Here structural analysis of hydroxyketoacid aldolase from Sphingomonas wittichii RW1 (SwHKA) revealed a dynamic movement of the metal cofactor between two coordination spheres without protein scaffold rearrangements. Holo‐SwHKA forms a trimer of homodimers, in which each monomer adopts an (α/β)8 triosephosphate isomerase (TIM) barrel fold. In total, holo‐SwHKA contains six equivalent active sites; each of which is formed from amino acids from two different domain‐swapped dimers. The transition from M2+ R to M2+ A,S is induced by bidentate substrate binding and occurs without a concomitant rearrangement of the protein scaffold.

To gain insight into the earlier observed activation of the enzyme by phosphate and a possible interaction thereof with the metal, phosphate was included into the crystallisation and soaking studies. Neither was the case for SwHKA. Docking studies did however reveal a potential docking site, close to H44 (Figure S6a&b). The docking does however support the earlier proposed function in the pyruvate deprotonation, studied by H/D exchange. In both cases 100–300 fold improved deprotonation rates were observed. This could be enabled by a phosphate in concert with H44.

>[2x]HHNKVRTCWNEGRPALAGWLQLPGTLHAEALARLDYDAVVIDMQASPIDFGQVAPMLIAIELGGAEPFVRTQVNDPSDIMKLLDAGAYGIIAPMVNTRAEAQTLASALHYSPRGLRSFGPRRPSLRYGSGYLAQASETVVGLAMIETREALANIDEILSVDGIDGVFIGPTDLALDLGHAPLVDTEEAEVVSAIAHVRERAHAAGKRVGIFCGSGGFARVKLAEGFDFVTAAPDLAMLSAAARQVIADARAL>MAWWKAWIEQEGVTVASSSHFNPDPDAETLYKAMKGIGTNEQAIIDVLTKRSNTQRQQIAKSFKAQFGKDLTETLKSELSGKFERLIVALMYPPYRYEAKELHDAMKGLGTKEGVIIEILASRTKNQLREIMKAYEEDYGSSLEEDIQADTSGYLERILVCLLQGSRDDVSSFVDPALALQDAQDLYAAGEKIRGTDEMKFITILCTRSATHLLRVFEEYEKIANKSIEDSIKSETHGSLEEAMLTVVKCTQNLHSYFAERLYYAMKGAGTRDGTLIRNIVSRSEIDLNLI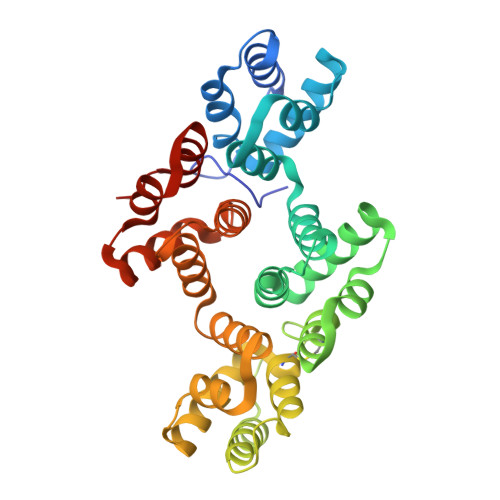KCHFKKMYGKTLSSMIMEDTSGDYKNALLSLVGSDP[2x]>[4x]GSAMGSASTSGNPFQANVEMKTFMERFNLTHHHQSGIYVDLGQDKEVDGTLYREPAGLCPIWGKHIELQQPDRPPYRNNFLEDVPTEKEYKQSGNPLPGGFNLNFVTPSGQRISPFPMELLEKNSNIKASTDLGRCAEFAFKTVAMDKNNKATKYRYPFVYDSKKRLCHILAVSMQLMEGKKYCSVKGEPPDLTWYCFKPRKSVT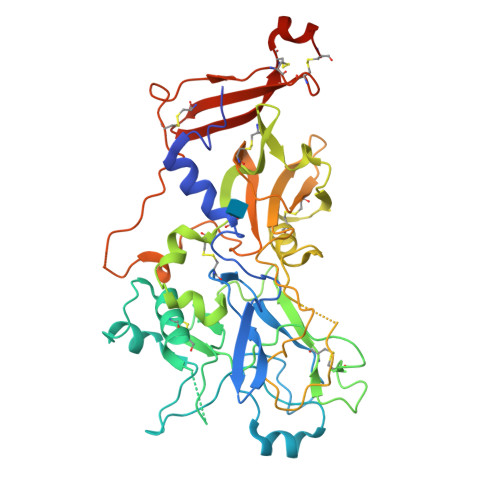ENHHLIYGSAYVGENPDAFISKCPNQALRGYRFGVWKKGRCLDYTELTDTVIERVESKAQCWVKTFENDGVASDQPHTYPLTSQASWNDWWPLHQSDQPHSGGVGRNYGFYYVDTTGEGKCALSDQVPDCLVSDSAAVSYTAAGSLSEETPNFIIPSNPSVTPPTPETALQCTADKFPDSFGACDVQACKRQKTSCVGGQIQSTSVDCTADEQNECGSNTAAALVPR> MYATMESVRLQSEAQQLAEMILQSETAENYRNCYKRLQEDEEAGRIIRS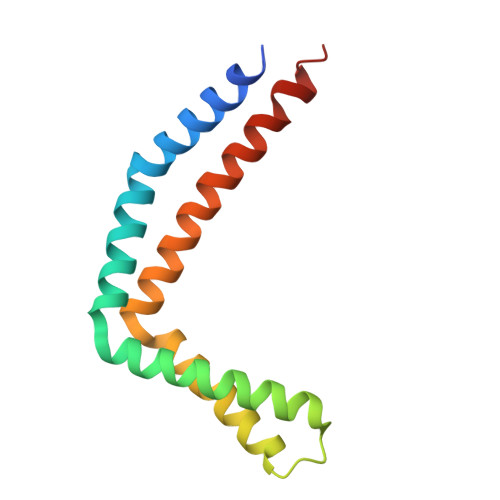FIKIKEQYEDVQRFGKYHPDYREISRKMREIKRELDLNDKVADFKRAENELQSILDEVSVEIGTAVSEHVKV>MPEGPELHLASQFVNEACRALVFGGCVEKSSVSRNPEVPFESSAYRISASARGKELRLILSPLPGAQPQQEPLALVFRFGMSGSFQLVPREELPRHAHLRFYTAPPGPRLALCFVDIRRFGRWDLGGKWQPGRGPCVLQEYQQFRENVLRNLADKAFDRPICEALLDQRFFNGIGNYLRAEILYRLKIPPFEKARSVLEALQQHRPSPELTLSQKIRTKLQNPDLLELCHSVPKEVVQLGGKGYGSESGEEDFAAFRAWLRCYGMPGMSSLQDRHGRTIWFQGD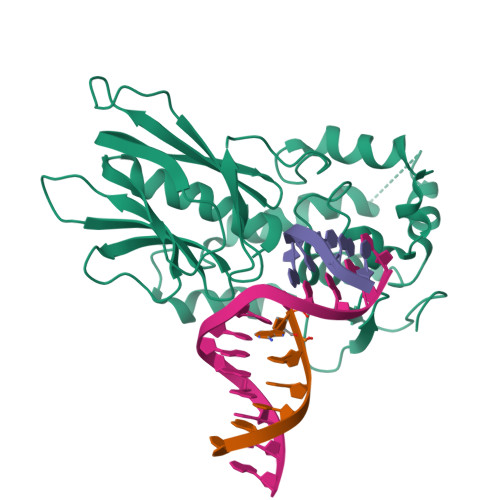PGPLAPKGRKS[2x]> MGSHHHHHHSQDPMAYSTREILLALCIRDSRVHGNGTLHPVLELAARETPLRLSPEDTVVLRYHVLLEEIIERNSETFT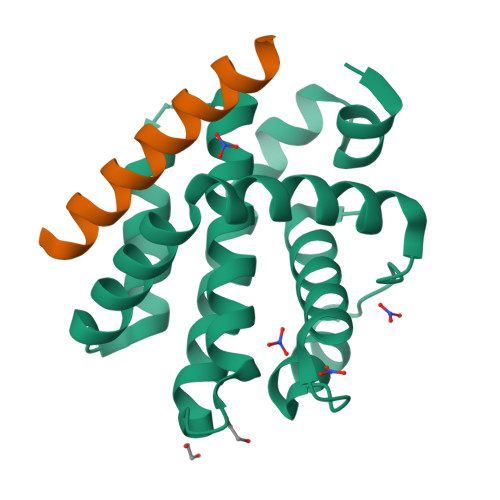ETWNRFITHTEHVDLDFNSVFLEIFHRGDPSLGRALAWMAWCMHACRTLCCNQSTPYYVVDLSVRGMLEASEGLDGWIHQQGGWSTLIEDNIPG;> PSSTMGQVGRQLAIIGDDINRRYDSE>[2x]PNSGTLALLLDEGSKQLPQAIIIGVKKGGTRALLEFLRVHPDVRAV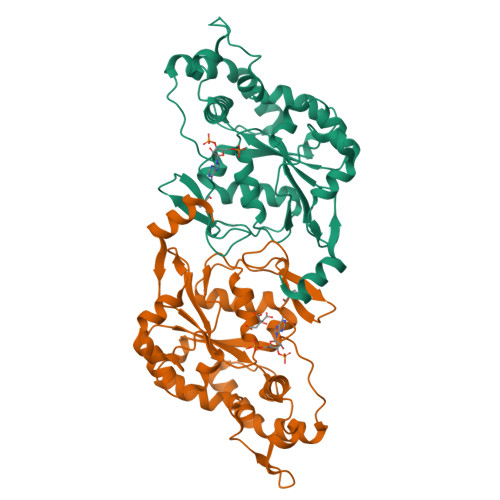GAEPHFFDRSYDKGLAWYRDLMPRTLDGQITMEKTPSYFVTREAPARISAMSKDTKLIVVVRDPVTRAISDYTQTLSKRPDIPTFESLTFKNRTAGLIDTSWSAIQIGIYAKHLEHWLRHFPIRQMLFVSGERLISDPAGELGRVQDFLGLKRIITDKHFYFNKTKGFPCLKKAEGSSRPHCLGKTKGRTHPEIDREVVRRLREFYRPFNLKFYQMTGHDFGWDG>GNEWEDEQYEQYVSFKAPIASGSDGVTTIYVRYKDNGKVTYQLPIIVSGSTVNSQDRDIHIAVDKDTLKTLNIERFSLYRPELWYTEMEEDKYEFPETVHIPAGSCVELLNIDFNLQDIDMLEKWVLPLTIVDDGSYAYQSHPR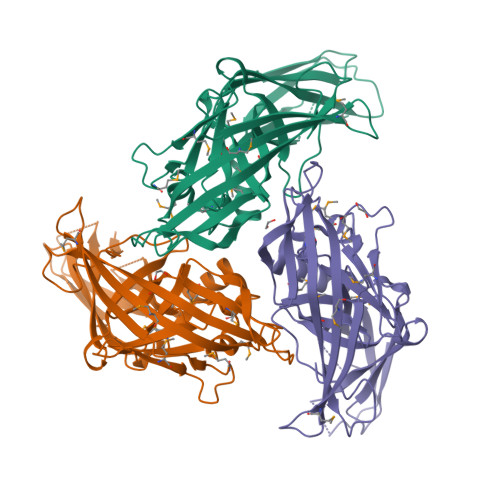KNYAKALLKVVPFNNYSGSYTASSMKVYTYINGKPDTNARTTDKRTGYVVDNNSIFFYAGLINEDMDKDMRKKYKINVHFKEDGTLDMKQDDPSNEMEFELIGTPTYSSTSVMDATRPYLERRYVQIMFEYDFQDFTYGGSGTEVIPIKYRVAGSMTLLRNINTQIPDEDQQIEW[6x]>[22x]HSQGTFTSDYSKYLDSRRAQ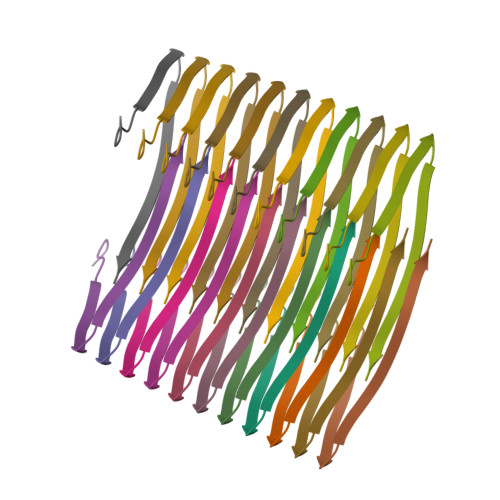DFVQWLMNT>[6x]GAMEMRLEKDRFSVNLDVKHFSPEELKVKVLGDVIEVHGKHEERQDEHGFISREFHRKYRIPADVDPLTITSSMSSDGVLTVNGPRKQVSGPER

Small Hsps (sHsps) form large oligomeric assemblies with a high capacity for holding onto nonnative proteins that are handed over to the ATP-driven chaperone machines for refolding. sHsps are ubiquitous among the kingdoms of life and within mammalian genomes occur in large families with members differentially expressed in many tissues including muscle, brain and the eye lens. Small Hsp sequences have in common an “α-crystallin domain” (ACD) of around 90 amino acids, with most having a short conserved C-terminal extension bearing an I-X-I motif and a longer variable N-terminal extension. The ACD is an immunoglobulin-like beta sandwich comprising strands β2–β9, and the assembly unit is a dimer. The conserved arginine in human sHsps is on the β6 + 7 strand at the dimer interface, not far from the dyad axis.

Here we have solved the X-ray structure of the ACD dimer of human αB R120G close to physiological pH, as well as higher-resolution αB ACD wild-type controls. Two mutations improved the diffraction resolution of crystals of human αB ACD: L137M substitution and truncation of the β2-strand. The sHsp wild-type ACD X-ray structures all have a deep groove that runs down the AP dimer interface. The groove is maintained through sequence changes, register shifts and across a wide pH range. The base of the groove is lined with four arginines, Arg120 and Arg116 on each of the β6 + 7 strands.> SRFADFFRN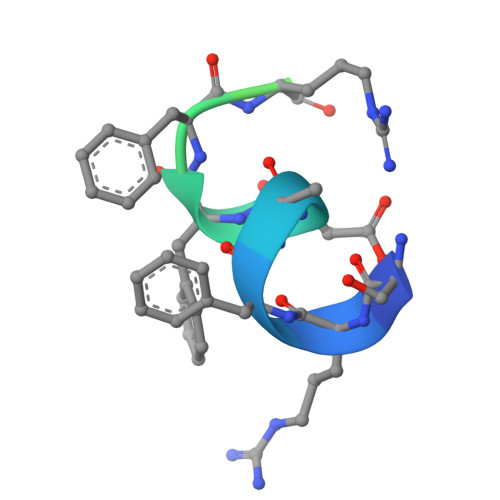EGLGSRSGSGK> KED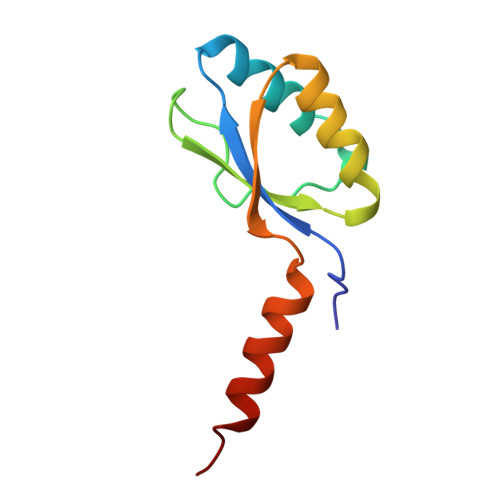FVGHQVLRITAADEAEVQTVKELEDLEHLQLDFWRGPGQPGSPIDVRVPFPSLQAVKVFLEAHGIRYRIMIEDVQSLLDEEQEQMFASQSR> MSGGLLKALRSDSYVELSQYRDQHFRGDNEEQEKLLKKS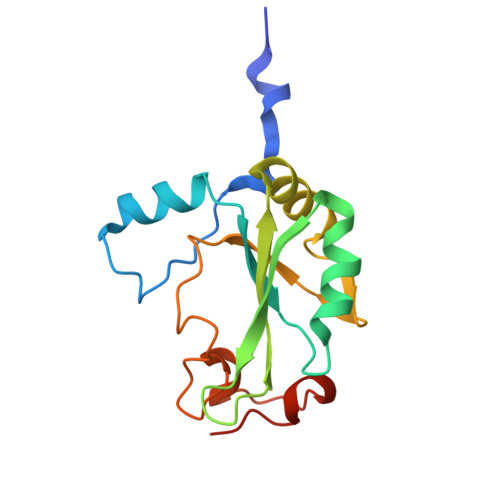CTLYVGNLSFYTTEEQIYELFSKSGDIKKIIMGLDKMKKTACGFCFVEYYSRADAENAMRYINGTRLDDRIIRTDWDAGFKEGRQYGRGRSGGQVRDEYRQDYDAGRGGYGKLAQNQ>[2x]EKPADSGPAVAQNTEYVGDEACKTCHSDVHSAWSETSHGNFIKDVTKDPKALPGNFEGNYPKMLNFKAEDIQYVLLGKPGALKVQELVGKKGTFGVPADDYPVMWASWDAGKGEWEIEVEAIGEGTPWLSTCAGCHVTGLTVPTDKNPKAAKAFAGFGITCEQCHGPGAKHIKNPQGEKMVISYDAENCGQCHSRGDSVAKTPDGKPFGYPYNDEGQYVPGKKLADYYTVVSVEGDKEGKLFWPTKHAKNSHHLQYPEWLMTGHATALETLKGNGHAQDRCLKCHSAEAYLAKEGTTVTMNDAKLGVTCQVCHASHDPAATKEAFLRKPKTEICTQCHNAEGGIVAGKEVHHPHKEMNEGKIGLGFPDSPSVMYKAGVTCVDCHMPKTAGPKASHLMKVVMPKDGKANGMPDSCSSCHPGASQDYLQNVIDTWQNDIKGRLAKVKAKLDAKKAAANSQAYKEALTYYSIVAADGSNGVHNYDLAVKLLTAAEQKLQKGELKLEGKPIPDPLLGLDSTRTGHHHHHH

In this paper, we describe the structural and functional properties of the nonaheme cytochrome OcwA, which is the terminal reductase of this organism. Surface-exposed OcwA is proposed to be the terminal reductase in T. potens JR extracellular electron transfer pathway, where it bridges the contact between bacterial metabolism and electrodes in MFC. We show that, in addition to solid electron acceptors, OcwA can also reduce soluble electron shuttles and oxyanions. Finally, rather than being a truncated member of the MtrC/OmcA/UndA protein family lacking one heme, OcwA is structurally related to NrfA, cytochrome c554, and MccA, which are key proteins in the nitrogen and sulfur cycles.

The three-dimensional (3D) structure of OcwA was determined to 2.2-Å resolution by X-ray crystallography. OcwA is composed by a globular heme domain and a three-helix bundle at the C terminus. These three long α-helices are reminiscent of the pentaheme NrfA (nitrite reductase) family of proteins and of the octaheme cytochromes hydroxylamine oxidoreductase (HAO) and sulfite reductase MccA. The crystal structure of OcwA shows that this protein forms a dimer, as observed experimentally by gel filtration. It spans about 180 by 81 by 45 Å but presents only limited contact (<2% of the total surface area) at the interface between monomers involving two regions. While the first contact area is formed by the base, but not the remainder, of the three-helix bundle, the second is made by a small alpha helix and a neighboring loop from an additional beta-sheet domain (amino acids 75 to 156) within the globular heme domain. The hemes in OcwA present three distinct coordination environments, as follows: hemes 1, 3, 4, 6, 7, and 8 (numbered according to the position of the CXXCH binding motif in the polypeptide sequence, where X is any amino acid) are bishistidine coordinated. Heme 9 features histidine-methionine coordination, whereas hemes 2 and 5 have histidine as a proximal ligand and an open coordination site at the distal position, thus being responsible for the EPR signal with a g value of 6. These two hemes, located at opposite ends of the nine-heme arrangement, have an almost identical environment, with a histidine serving as proximal iron ligand and a His-His motif (HH 281/282 at heme 2 and HH 380/381 at heme 5) situated above the distal face of the heme, which in both cases forms a solvent-exposed pocket. The organization of the hemes within OcwA, although vaguely reminiscent of the “staggered-cross” design of the structurally characterized outer membrane MHCs, clearly follows a different design that is similar to that of the NrfA family of proteins, with alternating parallel and perpendicular diheme packing motifs.> APSTTPVNEKATDAAKNLLSYLVEQAANGVTLSGQQDLESAQWVSDNVGKWPAILGIDFMDYSPSRVEYGAVGSTVPDAISYDSDGGIVTFCWHWGSPSGTYNTTDQPWWSNFYTEATAFDIAAAMDDPDSADYNLLVRDIDAISELLLQLQDLDIPILWRPLHQAEGGWFWWGAKGPEACIALYRLMFDRMTNHHGLNNLLWVWNSVDPSWYPGNDVVDIVSADIYADAGDHSPQEETFASLQSLTGDTKLVALGEVGNIPDPASTGGVADWAYWVTWNGDFIKGEDYNPLEYKKEVFSAENIITRDEVDV

Endo-β(1 → 4)-mannanases (endomannanases, EC 3.2.1.78) are important enzymes, catalysing the degradation of abundant plant β-mannans (hereafter mannan) in nature. Endomannanases catalyse cleavage of the β-(1 → 4)-linkages in mannans to produce mannooligosaccharides which may be further processed by e.g. the exo-acting β-mannosidases and α-galactosidases. Endomannanases from families 5, 26, and 113 belong to clan GH-A and share the (β/α)8-TIM barrel fold and catalytic machinery, and catalyse the cleavage of the O-glycosidic bonds in the mannan backbone with net retention of the anomeric configuration.

The structure of the deglycosylated YpenMan26A acid/base substituted variant E165Q, in complex with a α-62-61-di-galactosyl-mannotriose (MGG), was solved by molecular replacement using the known structure of PansMan26A24 as template, and refined at 1.36 Å resolution. The YpenMan26A chain can be traced from Ala1 to Val312 without breaks, and forms a (β/α)8-barrel fold as expected. The active site was identified in the groove with the conserved catalytic residue Glu165 (acid/base) mutated to Gln, and the conserved catalytic residue Glu257 (nucleophile), equivalent to those observed in PansMan26A24. Crystals of YpenMan26A E165Q were obtained in the presence of α-64-63-di-galactosyl-mannopentaose (MGGMM) with the aim that the oligosaccharide would span the catalytic site. However, the electron density of the ligand was modelled as MGG situated in the −4 to −2 subsites. Since YpenMan26A E165Q was not completely inactive, it is likely that the residual activity has caused hydrolysis of the MGGMM between the backbone monomers in the −1 and +1 subsites, after which MGG migrated to span the subsite −4 to −2, indicating high ligand affinity in these subsites. The electron density of MGG is clear and unambiguous, except for the galactopyranosyl unit in the −3 subsite, which points out of the binding cleft. There is electron density present near the mutated Q165, which is remote from the ligand, and was described as acetate, which fits the density well. There is a single N-glycosylation site at Asn103, located on the external side of the barrel, with a residual N-acetylglucosamine (GlcNac). Previously, enzyme interactions with a galactopyranosyl substituent attached to a mannopyranosyl unit within the −1 subsite of CjapMan26C have been described. Interestingly, because of the captured ligand in the present study, it is possible to identify interactions between the galactopyranose unit and the YpenMan26A in the −2 subsite not previously described.>GPLGRGREEKAPEEPQPVKMPENNSVVEATWNDVQLEDSLGMEVGYRLIPMVDFQQDGELLGRIRSIRKKFAQDMGFLPPVVHIRDNMDLQPARYRILMKGVEIGSGDAYPGRWLAI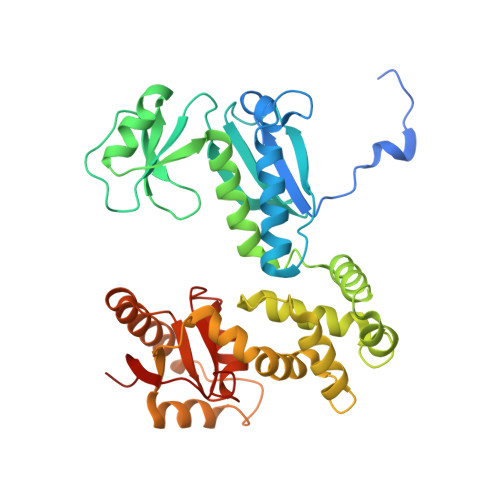NPGTAAGTLPGEKTVDPAFGLDAIWIESALKEQAQIQGFTVVEASTVVAMHLNHLIGQFSAELFGRQEAQQLLDRVSQEMPKLTEDLVPGVVTLTTLHKVLQNLLAEKVPIRDMRTILETLAEHAPLQSDPHELTAVVRVALGRAITQQWFPGNEEVQVIGLDTALERLLLQALQGGGGLEPGLADRLLAQTQEALSRQEMLGAPPVLLVNHALRPLLSRFLRRSLPQLVVLSNLELSDNRHIRMTATIGGK[2x]> RLETGNTVADISLGLINFLYSNFVPGGGFIVGLLELIWGFIGPSQWDIFLAQIEQLISQRIEEFARNQAISRLEGLSNLYKCYVRAFSDWEKDPTNPALRECMRIQFNDMNSALITAIPLFRVQNYEVALLSVYVQAANLHLSILRDVSVFGERWGYDTATINNRYSDLTSLIHVYTNHCVDTYNQGLRRLEGRFLSDWIVYNRFRRQLTISVLDIVAFFPNYDIRTYPIQTATQLTREVYLDLPFINENLSPAAVYPTFSAAESAIIRSPHLVDFLNSFTIYTDSLARSAYWGGHLVNSFRTGTTTNLIRSPLYGREGNTERPVTITASPSVPIFRTLSYPTGLDNSNPVAGIEGVEFQNTISRSIYRKSGPIDSFSELPPQDASVSPAIGYSHRLCHATFLERISGPRIAGTVFSWTHRSASPTNEVSPSRITQIPWVKAHTLASGASVIKGPGFTGGDILTRNSMGELGTLRVTFTGRLPQSYYIRFRYASVANRSGTFRYSQPPSYGISFPKTMDAGEPLTSRSFAHTTLFTPITFSRAQEEFDLYIQSGVYIDRIEFIPVTATFEAEYDLER

Two new modified Bacillus thuringiensis (Bt) proteins, Cry1Da_7 and Cry1B.868, with activity against fall armyworms (FAW), Spodoptera frugiperda (J.E. Smith), were evaluated for their potential to bind new insect receptors compared to proteins currently deployed as plant-incorporated protectants (PIPs) in row crops. Results from resistant insect bioassays, disabled insecticidal protein (DIP) bioassays, and cell-based assays using insect cells expressing individual receptors demonstrate that receptor utilizations of the newly modified Cry1Da_7 and Cry1B.868 proteins are distinct from each other and from those of commercially available Bt proteins such as Cry1F, Cry1A.105, Cry2Ab, and Vip3A. Accordingly, these two proteins target different insect proteins in FAW midgut cells and when pyramided together should provide durability in the field against this economically important pest. Taken together, these results support the conclusion that Cry1Da_7 and Cry1B.868 are effective insecticidal proteins against FAW that have the same pore-forming mode of action as other three-domain Bt proteins but bind to different receptors, suggesting that they would control resistance and increase product durability.

The Cry1Da_7 protein described here was identified by applying methods similar to those used for improving Cry51 against Lygus spp.. Cry1Da.844_8 containing the S282V, Y316S, and I368P amino acid substitutions exhibited a 50-fold improvement in activity toward CEW while maintaining toxicity toward FAW. The Cry1Da.844_8 and Cry1Da_7 proteins have 100% sequence identity in domains 1 to 3, and the full-length proteins were observed to readily undergo proteolysis using trypsin (data not shown). The resulting activated cores are comprised of the same pore-forming domain (D1) and same putative receptor biding domains (D2 and D3); correspondingly, their receptor utilizations were expected to be the same. The FAW activities of the Cry1Da_7 proteins with and without preproteolysis were comparable, suggesting that their PTX domains (domains 4 to 7) do not impact their stability or their receptor utilization in feeding assays. Consistent with this observation, the Cry1Da.844_8 and Cry1Da_7 proteins were also comparably active against FAW in insect feeding assays. There was no detectable difference in insect responses between the Cry1Fa-SS and Cry1Fa-RR colonies for both Cry1Da_7 and Cry1B.868, suggesting that the Cry1F-resistant colony was not cross-resistant to either Cry1Da_7 or Cry1B.868. Potential cross-resistance of Vip3A-resistant FAW to Cry1Da_7 and Cry1B.868 was also evaluated in comparative dose-response bioassays between susceptible (Vip3A-SS) and resistant (Vip3A-RR) colonies. Both Vip3A-SS and Vip3A-RR colonies were highly susceptible to the Cry1Da_7 protein, showing 50% lethal concentration (LC50) values of 11 and 12 ng/cm2, respectively, and all insects were dead at concentrations above 316 ng/cm2 Cry1Da_7 (data not shown).>MQKTLEVWIMPNSPQPAEDFKALVAPFEKAHGVEVKVTVLDAGVAWTKITTAATSGVGPDLTQLGTTWVGAISAMGVLEPVDDVLEALGGEKAYLPAVWRTTRLEGARQATAVPWFSELRAFYYRTDALKAAGVNPAEMFASWQGFEAGLARLKASSFRDPETKAPLAPLCTPGKNSWDVLHNAAPWIWGAGGEIVRQAGGRWQSALNSPESLEGLYFFLSLAQKGYVPAESLEKNTAQIEADFQAGKCAVFASGPWMIQRAQVPEAKGGFAERTAAKNLGVAPYPAGPKGRYTFFGGSNLALFNFSKNKPLAKELLKYLGGPEAQVRYAQMTGMLPALRSAWSDPSFQQNPLLRTFIQAAQFGRTYPSLAGWGGVENLAVQHLGMAWDLVAQGRL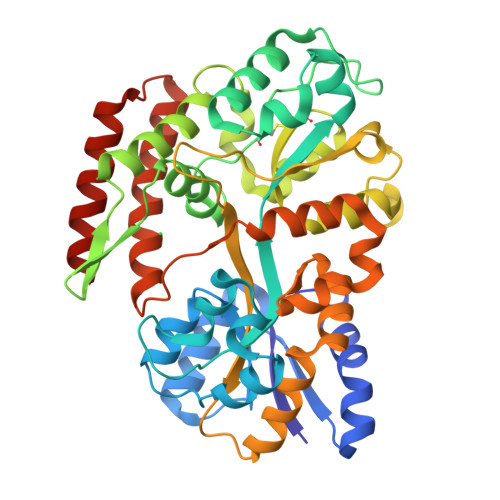TREALKDLMDKASAAINQALRHHHHHH[12x]>[2x]MGLAVFLPPYPFRGLKAPYLWMFYKYLHCATDSILFITGEDYLSVTDDEAQRARWEFDPASMASLGYELPNAQSMACHEYLTLDNA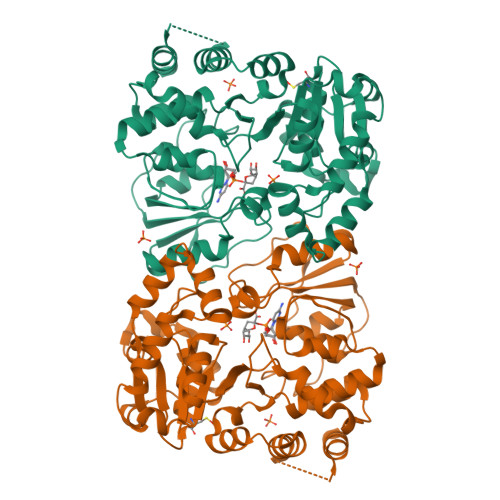FYETLLSRHHHDPIKSFSAFLTERIPDLETELHALLDSKKGIIDQIDTFISICNCPSLEHVARTLGKEVMHIEIGPLRAPMYRNTAYLDFAGVNGGTEASARYEKCQAEFDIKASLGDLHNYFLEVLPPAEAATHSAAGVVLQVEDNSNLIAYNHDFTNISLLSYVRQRYEKEDILVRAHPGSLFRLRDDVFTIDDSANSLAFINQCNEVFTINSSVGLEAILTGKKTTVLGDCSYAFINELAGASATVNAAAFYLFSYLVPFDLVFNQEYLKFRLGHPEEREIVGKHIEFYSADMPGSLSQAAHSLSSLINEAISLEHHHHHH> GAVEEDDKDKAKRVSRNKSEKKRRDQFNVLIKELGSMLPGNARKMDKSTVLQKSIDFLRKHKETTAQSDASEIRQDWKPTFLSNEEFTQLMLEALDGFFLAIMTDGSIIYVSESVTSLLEHLPSDLVDQSIFNFIPEGEHSEVYKILSTHLLESDSLTPEYLKSKNQLEFCCHMLRGTIDPKEPSTYEYVRFIGNFKSLTSVSTSTHNGFEGTIQRTHRPSYEDRVCFVATVRLATPQFIKEMCTVEEPN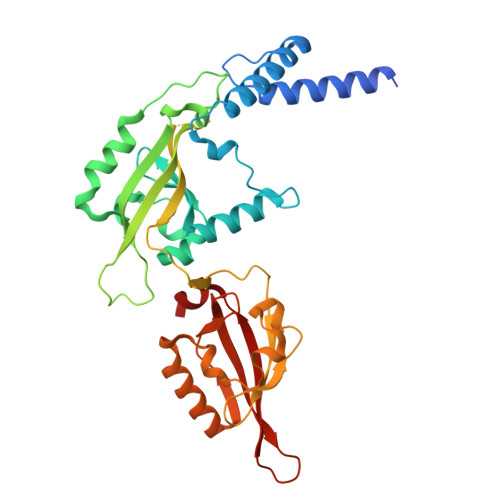EEFTSRHSLEWKFLFLDHRAPPIIGYLPFEVLGTSGYDYYHVDDLENLAKCHEHLMQYGKGKSCYYRFLTKGQQWIWLQTHYYITYHQWNSRPEFIVCTHTVVSYAEVRAE> NVNLEQLKQKAESGEAKAQLELGYRYFQGNETTKDLTQAMDWFRRAAEQGYTPAEYVLGLRYMNGEGVPQDYAQAVIWYKKAALKGLPQAQQNLGVMYHEGNGVKVDKAESVKWFRLAAEQGRDSGQQSMGDAYFEGDGVTRDYVMAREWYSKAAEQGNVWSCNQLGYMYSRGLGVERNDAISAQWYRKSATSGDELGQLHLADMYYFGIGVTQDYTQSRVLFSQSAEQGNSIAQFRLGYILEQGLAGAKEPLKALEWYRKSAEQGNSDGQYYLAHLYDKGAEGVAKNREQAISWYTKSAEQGDATAQANLGAIYFRLGSEEEHKKAVEWFRKAAAKGEKAAQFNLGNALLQGKGVKKDEQQAAIWMRKAAEQGLSAAQVQLGEIYYYGLGVERDYVQAWAWFDTASTNDMNLFGTENRNITEKKLTAKQLQQAELLSQQYIEKYAPEAWARMQKLKAQSAVKTGNK

The protein coded by locus c5321 from CFT073 E. coli was identified as one of nine potential vaccine candidates against ExPEC and was able to confer protection with an efficacy of 33% in a mouse model of sepsis. c5321 (known also as EsiB) lacks functional annotation and structurally belongs to the Sel1-like repeat (SLR) family. Structural domains composed of several such motifs are thought to act as interaction scaffolds to mediate protein-protein interactions. SLR-containing proteins are found in both prokaryotic (more prevalent) and eukaryotic organisms, and are thought to have been acquired by horizontal gene transfer. We have solved the structure of c5321 from uropathogenic Escherichia coli to 1.74 Å resolution. This antigen displays a super-helical Sel1-like repeat fold with eleven SLR units and a remarkably preserved consensus repeat sequence.

Here, we report the 1.74 Å-resolution crystal structure of c5321 from CFT073 E. coli determined by Se-Met SAD phasing. The crystallographic structure of the functional unit (aa 24–490) of c5321 has been solved by SAD phasing and refined to a resolution of 1.74 Å. The structure is composed of 11 SLR units, which to our knowledge represents the bacterial protein with the highest number of Sel1-like repeats solved up to date. The right-handed super-helix is approximately 115 Å in length, with a diameter of ~50 Å and a pitch (length of one complete helical turn measured parallel to the helix axes) of 60–65 Å. Electron density corresponding to a magnesium ion is identified in the c5321 structure, with the metal-ion-binding site located between repeats SLR3 and SLR4. Mg2+ coordination by residues of the intra-repeat loop, helix-1 and helix-1′ likely represents a means of stability/flexibility regulation in this region, for a currently unknown purpose. As the likely origin of the magnesium ion in the c5321 structure is MgCl2 used in the crystallization conditions, the natural metal ion for this system and its binding specificities remain to be determined. While disulfide bridges in HcpC lock the characteristic inter-repeat geometry, in c5321 a conserved tryptophan residue at repeat position 28 appears to contribute fundamentally in maintaining the same geometry by strengthening the inter-repeat hydrophobic core. Finally, the C-terminal region of the molecule contacts the C-terminal tail of the molecule in the adjacent asymmetric unit. Furthermore, crystal contacts observed between molecules belonging to neighbour asymmetric units share similarity to contacts characteristic for TPR-protein interactions with their physiological targets, suggesting a potential physiological interaction mode of c5321 with yet unidentified targets.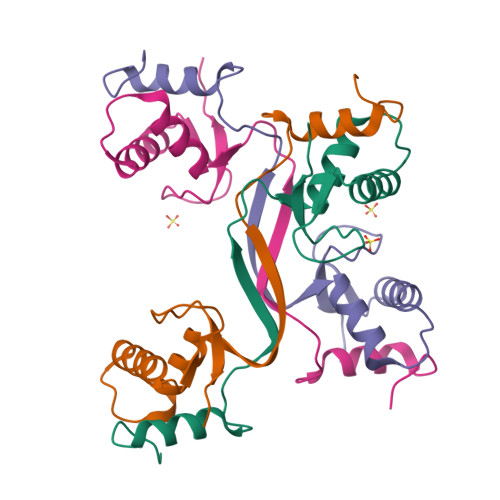>SSGLSVHTDMASVTKAMAAPESGLEVRDRMWLKITIPNAFLGSDVVDWLYHHVEGFPERREARKYASGLLKAGLIRHTVNKITFSEQCYYVFGDLSG[4x]>MGFLDGKRILLTGLLSNRSIAYGIAKACKREGAELAFTYVGDRFKDRITEFAAEFGSELVFPCDVADDAQIDALFASLKTHWDSLDGLVHSIGFAPREAIAGDFLDGLTRENFRIAHDISAYSFPALAKAALPMLSDDASLLTLSYLGAERAIPNYNTMGLAKAALEASVRYLAVSLGAKGVRVN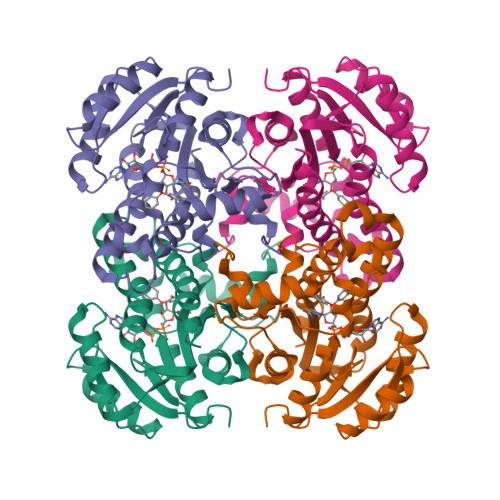AISAGPIKTLAASGIKSFGKILDFVESNSPLKRNVTIEQVGNAGAFLLSDLASGVTAEVMHVDSGFNAVVGGMAGLEEKLAAALEHHHHHH[3x]(1~{R},3~{S},5~{Z})-5-[(2~{E})-2-[(4~{a}~{R},5~{S},9~{a}~{S})-4~{a}-methyl-5-[(2~{R})-6-methyl-6-oxidanyl-heptan-2-yl]-3,4,5,6,7,8,9,9~{a}-octahydro-2~{H}-benzo[7]annulen-1-ylidene]ethylidene]-4-methylidene-cyclohexane-1,3-diol | C29 H48 O3 | 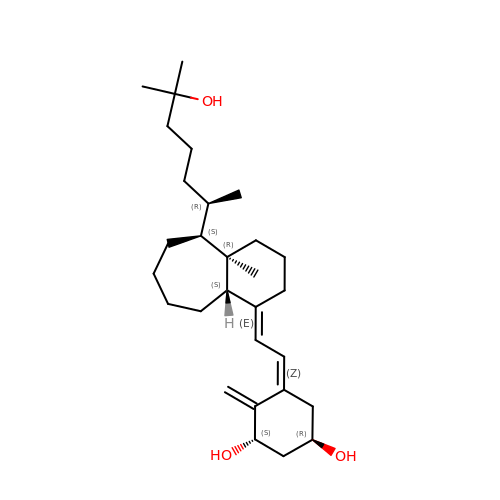XFWLTCCEILSQTJ-XDCKQIGSSA-N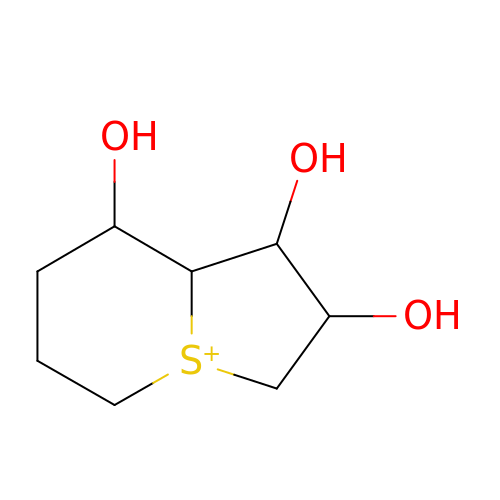(1R,5S,6S,7R,8S)-1-THIONIABICYCLO[4.3.0]NONAN-5,7,8-TRIOL | C8 H15 O3 S | YXHBFMXISHCSIQ-OZFRBSTCSA-N2-[(2E)-3-[(4-azanyl-2-methyl-pyrimidin-5-yl)methyl]-4-methyl-2-(1-oxidanylpropylidene)-1,3-thiazol-5-yl]ethyl phosphono hydrogen phosphate | C15 H24 N4 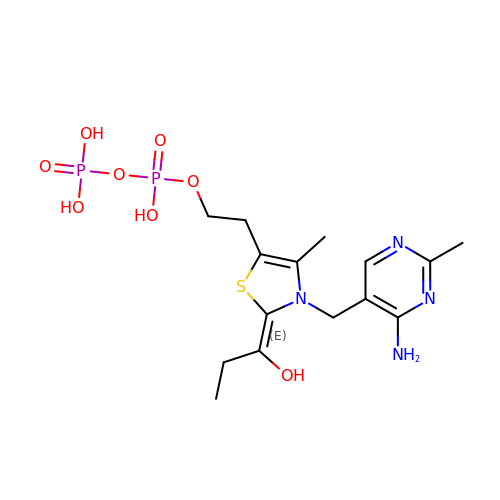O8 P2 S | MLWWWBMKISFTSY-NTCAYCPXSA-N ANILINE | 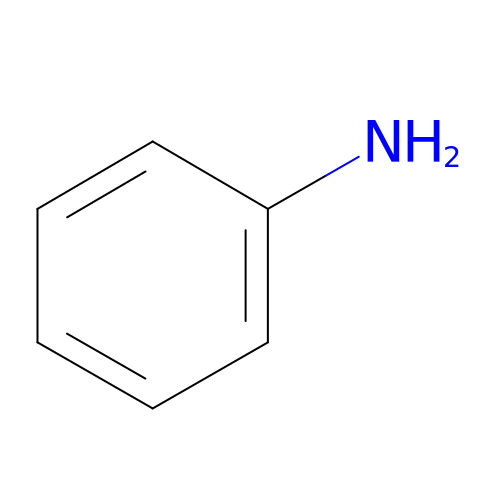C6 H7 N | PAYRUJLWNCNPSJ-UHFFFAOYSA-N> MAAQIPESDQIKQFKEFL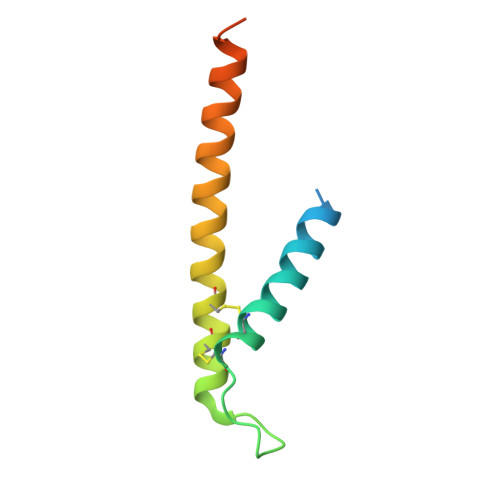GTYNKLTETCFLDCVKDFTTREVKPEETTCSEHCLQKYLKMTQRISMRFQEYHIQQNEALAAKAGLLGQPR> AAPQNLTTVPLTTIYECPPSPVKEIFS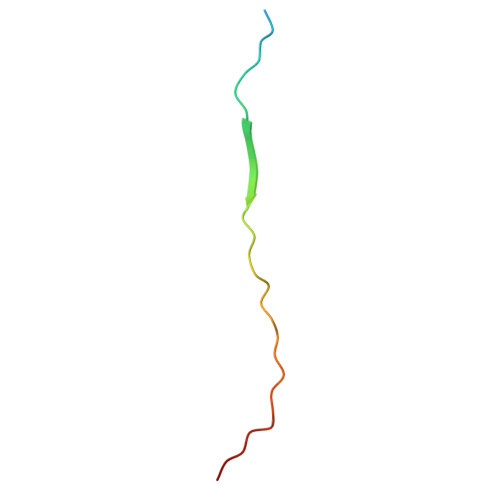YSKGIQTQ> GAMGSMSAPSSVPPHKMANLHKLQRAWTLWYDSPSTYNTENWEMSLVPIMTVHSVEEFFVMLRYMKPLHALRTSSQYHFFQEGVKPMWEDPANKKGGKLWVNLDITSANGR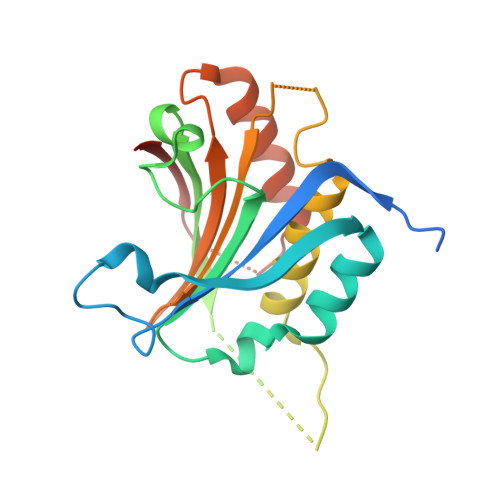SSNNNTSGTSAADGSAAEAKTDLDKAWENVLMATVGEYLDCVDKKDTPTEPFVTGIVMSKRKYHNRLAVWVSDASATDKIEALKKALTKEASLAPIASMVFTKHGEAS> ASITGDALVALPEGESVRIADIVPGARPNSDNAIDLKVLDR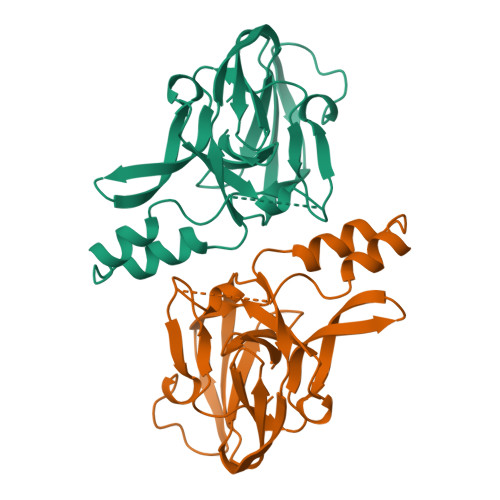HGNPVLADRLFHSGEHPVYAVRTVEGLRVTGTANHPLLCLVDVAGVPTLLWKLIDEIKPGDYAVIQRSAFSVDCAGFARGKPEFAPTTYTVGVPGLVRFLEAHHRDPDAKAIADELTDGRFYYAKVASVTDAGVQPVYSLRVDTADHAFITNGFVSHN> CGC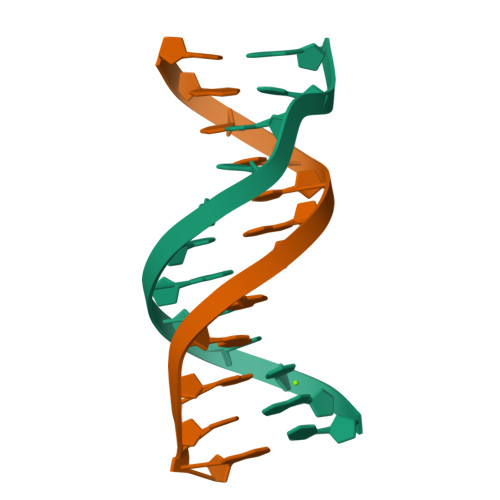TTATATGCG;> CGCATATAAGCG> GIDPFTKSELAVEILEKGQVRFWMQAEKLSGNAKVNYIFNEKEIFEGPKYKMHIDRNTGIIEMFMEKLQDEDEGTYTFQLQDGKATNHST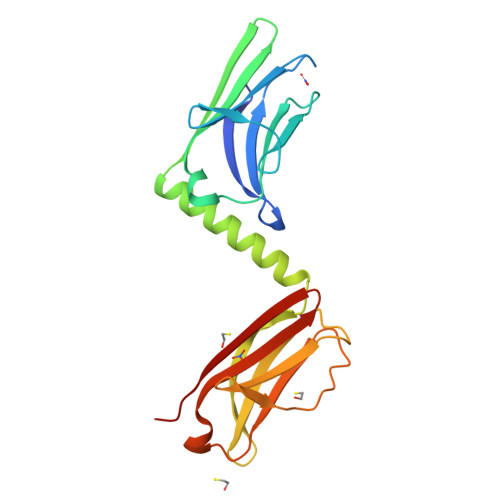VVLVGDVFKKLQKEAEFQRQEWIRKQGPHFVEYLSWEVTGECNVLLKCKVANIKKETHIVWYKDEREISVDEKHDFKDGICTLLITEFSKKDAGIYEVILKDDRGKDKSRLKLVDEA(3S)-6-cyclohexyl-3-{3-[(dimethylamino)methyl]-1,2,4-oxadiazol-5-yl}-N-hydroxyhexanamide 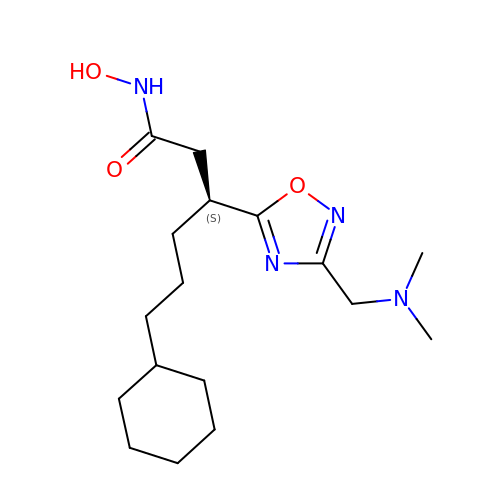| C17 H30 N4 O3 | ILYORWQDLYKJJF-AWEZNQCLSA-N Subsequently, the pathway involving aromatic aldehyde synthase, monoamine oxidase, and aldehyde dehydrogenase (AMA pathway) is introduced into E. coli Lys5 to produce glutarate from glucose. Module I contained two enzymes for converting lysine to glutaraldehyde, while Module II contained the last enzyme for converting glutaraldehyde to glutarate. In this study, an aldehyde dehydrogenase, ALDH, was isolated from K. pneumoniae to demonstrate its double oxidation capability. The simultaneous catalysis of the two aldehyde groups was verified through both experimental and mechanistic calculation methods, providing a enzyme that extends the existing aldehyde dehydrogenase library.

ALDH was identified as the rate-limiting enzyme in the AMA pathway based on three experiments: (i) Enzyme activity assay: Despite being more highly expressed than the other two enzymes, ALDH exhibited the lowest enzyme activity. Subsequently, ALDH was crystallized to obtain the protein crystal structure with a resolution of 2.28 Å. Each ALDH monomer was found to comprise three domains: an oligomerization domain, a catalytic domain, and an NAD+-binding domain. The ternary conformation was determined by molecular docking of the substrate glutaraldehyde and cofactor NAD+ with ALDH. Based on the catalytic mechanism of aldehyde dehydrogenase on single-aldehyde substrates, a putative catalytic mechanism of ALDH was proposed: Tyr-88 initiates a nucleophilic attack on the carbonyl group of glutaraldehyde; Subsequently, the hydrogen (H) on the synthesized hemiacetal hydroxyl (OH) is deprotonated. Simultaneously, the hydrogen (H) on the central carbon of the hemiacetal is transferred from the substrate to the carbon of the amide neighbor of the cofactor NAD+; Finally, the ester bond is hydrolyzed, resulting in the formation of glutarates. Our findings indicated that the reaction could not proceed under acidic conditions; and (iv) Key residue validation: When Tyr88 residue was mutated to alanine, its catalytic efficiency was significantly reduced, nearly reaching zero. The high energy potentials of steps 2 and 5 were caused by the suboptimal orientation of IN1 and IN4 toward the cofactor NAD+. Whole-cell conversion of Mu4 produced 9.9 g/L of glutarate, which was 4.0-fold than that produced by wild-type ALDH. Finally, the above mutant sites were combined to generate the mutant Mu5 (ALDHI90C/I212C/N94S/P95N/G210T), capable of producing 13.9 g/L glutarate from 20 g/L glutaraldehyde in 30 h, representing a 5.6-fold improvement over wild-type ALDH. The increase in the catalytic activity of the Mu5 mutant could be explained in three ways: (i) The k cat, K M, and k cat/K M values of Mu5 were 27.9-fold, 1.5-fold, and 51.0-fold compared to the corresponding values for wild-type ALDH.

>[2x]RGSMTIQDIQSLAEAHGLLLTDKMNFNEMGIDFKVVFALDTKGQQWLLRIPRRDGMREQIKKEKRILELVKKHLSVEVPDWRISSTELVAYPILKDNPVLNLDAETYEIIWNMDKDSPKYITSLAKTLFEIHSIPEKEVRENDLKIMKPSDLRPEIANNLQLVKSEIGISEQLETRYRKWLDNDVLWADFTQFIHGDLYAGHVLASKDGAVSGVIDWSTAHIDDPAIDFAGHVTLFGEESLKTLIIEYEKLGGKVWNKLYEQTLERAAASPLMYGLFALETQNESLIVGAKAQLGVI> MGDSILSQAEIDALLNGDSDTKDEPTPGIASDSDIRPYDPNTQRRVVRERLQALEIINERFARQFRMGLFNLLRRSPDITVGAIRIQPYHEFARNLPVPTNLNLIHLKPLRGTGLVVFSPSLVFIAVDNLFGGDGRFPTKVEGREFTHTEQRVINRMLKLALEGYSDAWKAINPLEVEYVRSEMQVKFTNITTSPNDIVVNTPFHVEIGNLTGEFNICLPFSMIEPLRELLVNPPLENSRHEDQNWRDNLVRQVQHSELELVANFADIPLRLSQILKLKPGDVLPIEKPDRIIAHVDGVPVLTSQYGTVNGQYALRVEHLIN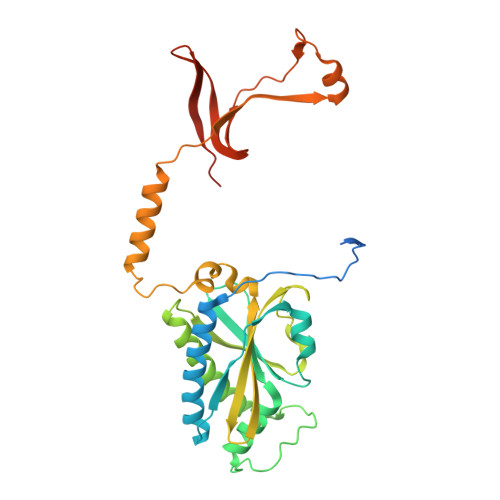PILNSLNEEQPK5-chloranyl-6-[1-[(3-fluorophenyl)methyl]pyrazol-4-yl]pyrimidin-4-amine | C14 H11 Cl F N5 | 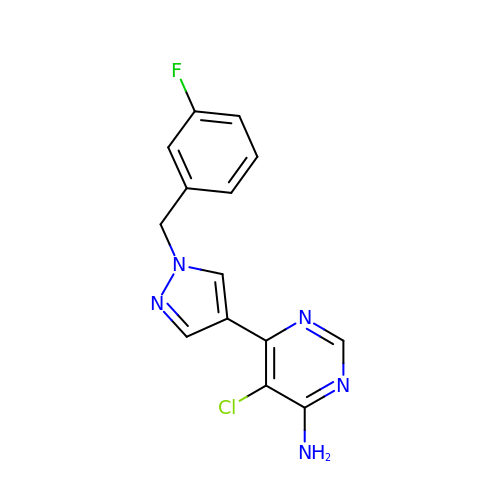SAVYHHAWTAHFAW-UHFFFAOYSA-N>GPGSMAGAIASRMSFSSLKRKQPKTFTVRIVTMDAEMEFNCEMKWKGKDLFDLVCRTLGLRETWFFGLQYTIKDTVAWLKMDKKVLDHDVSKEEPVTFHFLAKFYPENAEEELVQEITQHLFFLQVKKQILDEKVYCPPEASVLLASYAVQAKYGDYDPSVHKRGFLAQEELLPKRVINLYQMTPEMWEERITAWYAEHRGRARDEAEMEYLKIAQDLEMYGVNYFTIRNKKGTELLLGVDALGLHIYDPENRLTPKISFPWNEIRNISYSDKEFTIKPLDKKIDVFKFNSSKLRVNKLILQLCIGNHDLFMRRRKADS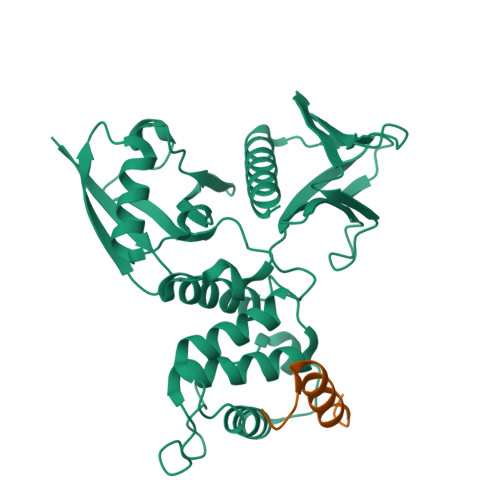LEVQQ[4x];>PKFGTHHKALQEIRNSLLPFANETNSSRSTSE[4x]> MGSSHHHHHHSSGLVPRGSSMEMIEKAPTDLEDRDKAPHLLLLAGIHGDEPGGFNATNLFLMHYSVLKGLVEVVPVLNKPSMLRNHRGLYGDMNRKFAALDKKDPEYPTIQEIKSLIAKPNIDAVLHLHDGGGYYRPVYVDAMLNPKRWGNCFIIDQDEVKGAKFPNLLAFANNTIESINAHLLHPIEEYHLKNTRTAQGDTEMQKALTFYAINQKKSAFANEASKELPLASRVFYHLQAIEGLLNQLNIPFKRDFELNPSSVHALINDKSLWAKISSLPKIPLFNLRPRLNHFPLPHNTKIPQIPIESNAYIVGLVKNKQEVFLKYGNKLMTRLSPFYIEFDPSLEEVKMQIDNKDQMVKIGSVVEVKESFYIHAMDNIRANVIGFSVSNENKPNEAGYTIRFKDFQKRFSLDKQERIYRIEFY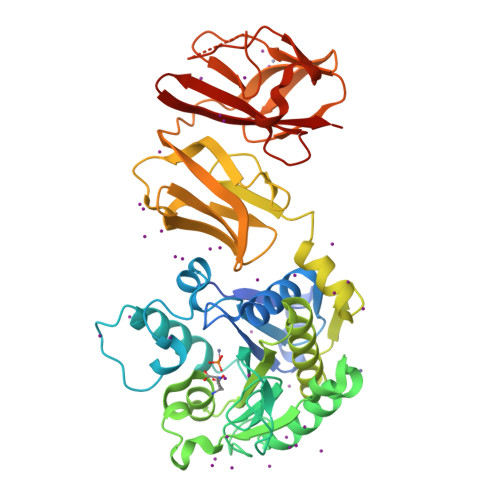KNNAFSGMILVKFV> MKNNKIYLLGACLLCAVTTFAQNVSLQPPPQQLIVQNKTIDLPAVYQLNGGEEANPHAVKVLKELLSGKQSSKKGMLISIGEKGDKSVRKYSRQIPDHKEGYYLSVNEKEIVLAGNDERGTYYALQTFAQLLKDGKLPEVEIKDYPSVRYRGVVEGFYGTPWSHQARLSQLKFYGKNKMNTYIYGPKDDPYHSAPNWRLPYPDKEAAQLQELVAVANENEVDFVWAIHPGQDIKWNKEDRDLLLAKFEKMYQLGVRSFAVFFNDISGEGTNPQKQAELLNYIDEKFAQVKPDINQLVMCPTEYNKSWSNPNGNYLTTLGDKLNPSIQIMWTGDRVISDITRDGISWINERIKRPAYIWWNFPVSDYVRDHLLLGPVYGNDTTIAKEMSGFVTNPMEHAESSKIAIYSVASYAWNPAKYDTWQTWKDAIRTILPSAAEELECFAMHNSDLGPNGHGYRREESMDIQPAAERFLK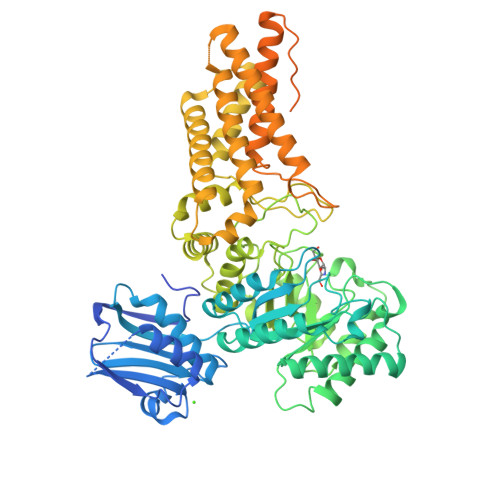AFKEGKNYDKADFETLQYTFERMKESADILLMNTENKPLIVEITPWVHQFKLTAEMGEEVLKMVEGRNESYFLRKYNHVKALQQQMFYIDQTSNQNPYQPGVKTATRVIKPLIDRTFATVVKFFNQKFNAHLDATTDYMPHKMISNVEQIKNLPLQVKANRVLISPANEVVKWAAGNSVEIELDAIYPGENIQINFGKDAPCTWGRLEISTDGKEWKTVDLKQKESRLSAGLQKAPVKFVRFTNVSDEEQQVYLRQFVLTIEKK> MAHHHHHHMKITYCDALIIGGGLAGLRASIACKQKGLNTIVLSLVPVRRSHSAAAQGGMQASLANAKKSEGDNEDLHFLDTVKGSDWGCDQQVARMFVTTAPKAIRELASWGVPWTRIKKGDRPAVVNGEHVIITERDDRHGYILSRDFGGTKKWRTCFTADATGHTMLYAVANEALHHKVDIQDRKDMLAFIHHDNKCYGAVVRDLITGEISAYVSKGTLLATGGYGRVYKHTTNAVICDGAGAASALETGVAKLGNMEAVQFHPTALVPSGILMTEGCRGDGGVLRDKFGRRFMPAYEPEKKELASRDVVSRRILEHIQKGYGAKSPYGDHVWLDIAILGRNHVEKNLRDVRDIAMTFAGIDPADSEEQTKDNMQGMPANEPEYGQAMAKQKGWIPIKPMQHYSMGGVRTNPKGETHLKGLFCAGEAACWDLHGFNRLGGNSVSEAVVAGMIIGDYFASHCLEAQIEINTQKVEAFIKESQDYMHFLLHNEGKEDVYEIRER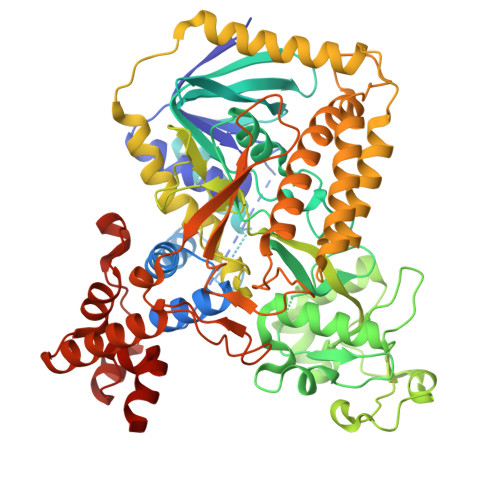MKEVMDEKVGVFREGKKLEEALKELQELYARSKNICVKNKVLHNNPELEDAYRTKKMLKLALCITQGALLRTESRGAHTRIDYPKRDDEKWLNRTLASWPSTEQDMPTIEYEELDVMKMEISPDFRGYGKKGNFIPHPKKEERDAEILKTILELEKLGKDRIEVQHALMPFELQEKYKARNMRLEDEEVRARGEHLYSFNVHDLLDQHNANLKGEHHE> MARKTKQEAQETRQHILDVALRLFSQQGVSSTSLGEIAKAAGVTRGAIYWHFKDKSDLFSEIWELSESNIGELELEYQAKFPGDPLSVLREILIHVLESTVTEERRRLLMEIIFHKCEFVGEMAVVQQAQRNLCLESYDRIEQTLKHCIEAKMLPADLM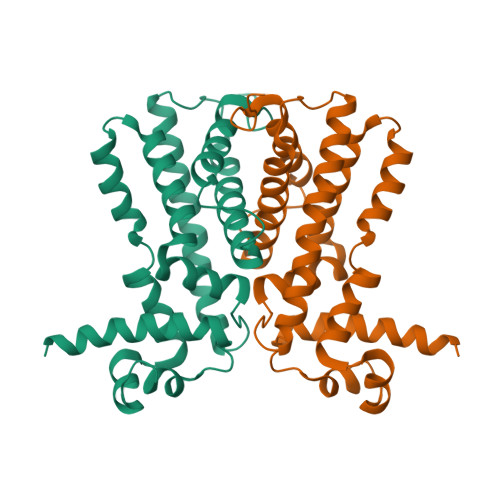TRRAAIIMRGYISGLMENWLFAPQSFDLKKEARDYVAILLEMYLLCPTLRNPATNE> MGSSHHHHHHSQDPNSMPDNTIQWDKDADGIVTLTMDDPSGSTNVMNEAYIESMGKAVDRLVAEKDSITGVVVASAKKTFFAGGDVKTMIQARPEDAGDVFNTVETIKRQLRTLETLGKPVVAAINGAALGGGLEIALACHHRIAADVKGSQLGLPEVTLGLLPGGGGVTRTVRMFGIQNAFVSVLAQGTRFKPAKAKEIGLVDELVATVEELVPAAKAWIKEELKANPDGAGVQPWDKKGYKMPGGTPSSPGLAAILPSFPSNLRKQLKGAPMPAPRAILAAAVEGAQVDFDTASRIESRYFASLVTGQVAKNMMQAFFFDLQAINAGGSRPEGIGKTPIKRIGVLGAGMMGAGIAYVSAKAGYEVVLKDVSLEAAAKGKGYSEKLEAKALERGRTTQERSDALLARITPTADAADFKGVDFVIEAVFENQELKHKVFGEIEDIVEPNAILGSNTSTLPITGLATGVKRQEDFIGIAFFSPVDKMPLVEIIKGEKTSDEALARVFDYTLAIGKTPIVVNDSRGFFTSRVIGTFVNEALAMLGEGVEPASIEQAGSQAGYPAPPLQLSDELNLELMHKIAVATRKGVEDAGGTYQPHPAEAVVEKMIELGRSGRLKGAGFYEYADGKR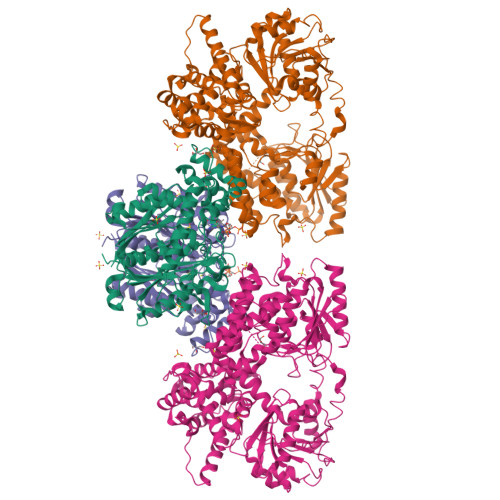SGLWPGLRETFKSGSSQPPLQDMIDRMLFAEALETQKCLDEGVLTSTADANIGSIMGIGFPPWTGGSAQFIVGYSGPAGTGKAAFVARARELAAAYGDRFLPPESLLS;> MSEEAFIYEAIRTPRGKQKNGSLHEVKPLSLVVGLIDELRKRHPDLDENLISDVILGCVSPVGDQGGDIARAAVLASGMPVTSGGVQLNRFCASGLEAVNTAAQKVRSGWDDLVLAGGVESMSRVPMGSDGGAMGLDPATNYDVMFVPQSIGADLIATIEGFSREDVDAYALRSQQKAAEAWSGGYFAKSVVPVRDQNGLLILDHDEHMRPDTTKEGLAKLKPAFEGLAALGGFDDVALQKYHWVEKINHVHTGGNSSGIVDGAALVMIGSAAAGKLQGLTPRARIVATATSGADPVIMLTGPTPATRKVLDRAGLTVDDIDLFELNEAFASVVLKFQKDLNIPDEKLNVNGGAIAMGHPLGATGAMILGTMVDELERRNARRALITLCIGGGMGVATIIERV PBP6b (also known as DacD) is another putative DD-CPase in E. coli, with 47% sequence identity to both PBP5 and PBP6a. PBP5, PBP6a, and PBP6b are periplasmic proteins binding to the cytoplasmic membrane by a C-terminal amphiphilic α-helix, which is important for the physiological function of PBP5 (33). Adjacent to the membrane anchor, there is an elongated, β-sheet-rich domain, which appears to position the globular, catalytic domain at a fixed distance from the membrane. Taken together, our data indicate that PBP6b is a DD-CPase specialized for growth at acidic pH and that the redundancy of DD-CPases ensures that sufficient activity is available under various pH conditions.

The construct that yielded crystals suitable for structure determination (PBP6bΔC) lacked the N-terminal 21 residues of the signal peptide and the C-terminal 14-residue membrane anchor. The structure of PBP6bΔC comprises two domains; the CPase domain is formed of residues Glu2 to Thr262, whereas the C-terminal domain comprises Thr263 to Thr346, with two breaks in the modeled polypeptide chain, between residues Lys272 and Asp287 and between residues Leu317 and Pro320, because of disorder. The crystals contain two PBP6bΔC copies per asymmetric unit, which can be superimposed with the root mean square deviation (RMSD) of 0.3 Å on 324 aligned Cα atoms. There is no significant difference in the relative dispositions of the two domains in the two molecules in the asymmetric unit, therefore, the two chains can be considered to be essentially identical. Given the 48% sequence identity between the PBP6b and PBP5, it is unsurprising that the structures of PBP6bΔC and various PBP5ΔC constructs superimpose well. A global superimposition of 292 Cαs yields an RMSD value of 1.4 Å, indicating that the relative dispositions of the two domains in each PBP are the same. Despite cocrystallization of PBP6bΔC with 2 mM diacetyl-l-Lys-d-Ala-d-Ala, there is no evidence of bound product from the pseudosubstrate. The crystal packing involves the region immediately surrounding the PBP6bΔC active site (Ser42) such that the observed crystal packing would likely have been disfavored had the product of the CPase reaction been bound. Of all the residues within 10 Å of the Ser42 side chain hydroxyl, all but one are invariant between PBP6bΔC (Asn39) and PBP5 (Asp49). Asn39 in PBP6bΔC is 9 Å away from the nucleophilic Ser42, and, should the CPase reaction proceed using a Grotthuss-like proton relay mechanism similar to that of the GH45 cellulase, residues His214 and Ser216 are likely intermediates between Ser42 and Asn39.

>[2x]MGSSHHHHHHSSGENLYFQGHMAENIPFSPQPPEIHAGSWVLMDYTTGQILTAGNEHQQRNPASLTKLMTGYVVDRAIDSHRITPDDIVTVGRDAWAKDNPVFVGSSLMFLKEGDRVSVRDLSRGLIVDSGNDACVALADYIAGGQRQFVEMMNNYAEKLHLKDTHFETVHGLDAPGQHSSAYDLAVLSRAIIHGEPEFYHMYSEKSLTWNGITQQNRNGLLWDKTMNVDGLKTGHTSGAGFNLIASAVDGQRRLIAVVMGADSAKGREEEARKLLRWGQQNFTTVQILHRGKKVGTERIWYGDKENIDLGTEQEFWMVLPKAEIPHIKAKYTLDGKELTAPISAHQRVGEIELYDRDKQVAHWPLVTLESVGEG> MASKKGTDAPAALTDPLKEDPTVIRDEAQFPEPSLYFKVFESEAGEPEAKIRADVNKLYDRWIEKYGRRWPEDGINTEDMVWLAEEANKRKRAKPRPRGTVAAEKTEYEDEFMPDPTVGAPVSAADAAKAARRAKKDRKKKKAAGGAEQPAGPRTNYEKTVAGGKWVTDEFESADYEAGNLEKLWDMYLWDREGKPTMMPDTPAAQQEGEESEDFDDFYTAYRPRDVDSEEAREAVWATDEFESDEDNTESEWAPEYVGAGLGLVAEDPLNPQYSLRHSNHPLAPFPGEPLKWASYVYPDFTTFEGLSKQSIPHGMGVMTFGTGTGAGFAMSQTRYGDKYEGEFQAGYAHGLGQFTSEASGEVYIGEFFAGQRHGCGMTLDMKPYFYLLERGVDPVEAYRRTAGAIMKNVEVRT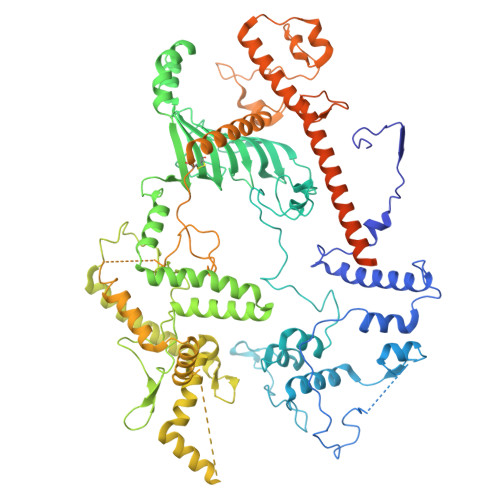WYRGNKLGDAKEDEVVEINVLKDELDDPFEIALRNSLHDAKLRKWKAMSPQDKAMDRIVSIIERVQRRNPGRFGAYYREDEKGRVRPVLDSDGADTDFDSVDMIQGVDTDGDLGPGWEGATDSEENPMDPRIRELMAAEGMDDKLEDEGFKDTVLGSAIINPYTGLDMKTYLDGKERHQAELVSVYKASREGRKYLNKVRKDKGGAAKDDESSYVEDDAASGHPGALLSREAEDDRLARLYEQAGVSKEDERRVEGLAARWRRLLAADEEEVLGGAVGAFRRPGNPLAANDSDTGFETESDMMEMCDIPEILGTVQEARQIVERARMWRFKPYGEVGLRMAQDANGSPVSLMQEPLHYPHGTKFMAPGPLGLCHAVPDDPSLRQEMAKVAHNYAAIYRMYNFDWDPEPGTVQYKIDQRIRRAQELRNNAMARYLAAADEVLRDGAAPAGEGDQALLLASTSTGAPEAFDGQGNASGSGSSSALSSRGGSMFASMTLSRPAPMAGVVSLGRAARVVLGAFADAAKSVPMARPRLARPSGRRQ>[4x]MAKILCVLYDDPITGYPKSYARADVPKIDHYPGGQTAPTPKQIDFTPGELLGSVSGELGLRKYLEGLGHTLVVTSDKEGEDSVFERELPDAEIVISQPFWPAYLTPERIAKAKKLKLAVTAGIGSDHVDLEAAIKNGITVAEV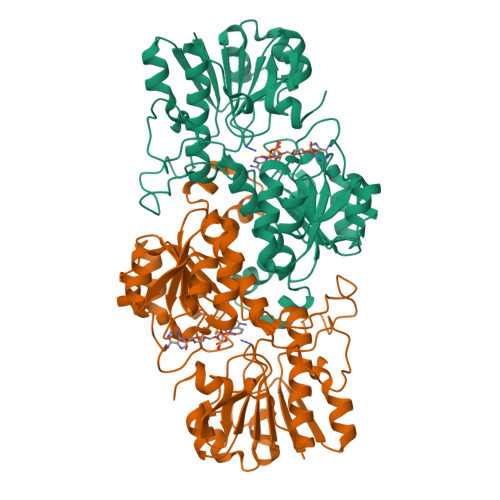TYSNSISVSEHVVMMILSLVRNYIPSYQWVIKGGWNIADCVERSYDLEAMHVGTVAAGRIGLAVLKRLKPFDVKLHYFARHRLPESVENELGLTYHPSVEDMVKVCDVVTINAPLHPGTLDLFNDELISKMKRGAYLVNTARGKICNRDAVVRALESGQLAGYAGDVWFPQPAPKDHPWRTMPHHGMTPHISGTSLSAQARYAAGTREILECWFEERPIREEYLIVDGGKLAGTGAHSYTVSK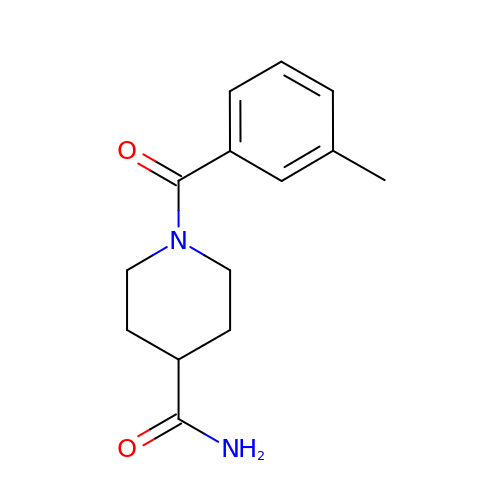1-(3-methylbenzene-1-carbonyl)piperidine-4-carboxamide | C14 H18 N2 O2 | VSYPROQBASLXDK-UHFFFAOYSA-N>[7x]SAAWEDEDLDTDNDNIPDAYEKNGYTIKDSIAVKWNDSFAEQGYKKYVSSYLESNTAGDPYTDYQKASGSIDKAIKLEARDPLVAAYPVVGVGMENLIISTNEHASSDQGKTVSRATTNSKTDANTVGVSISAGYQNGFTGNITTSYSHTTDNSTAVQ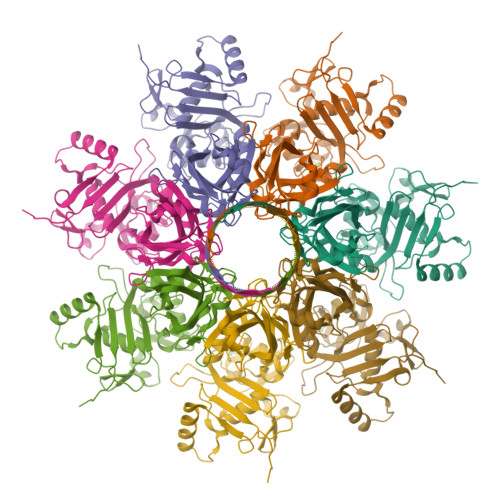DSNGESWNTGLSINKGESAYINANVRYYNTGTAPMYKVTPTTNLVLDGETLATIKAQDNQIGNNLSPNETYPKKGLSPLALNTMDQFNARLIPINYDQLKKLDSGKQIKLETTQVSGNYGTKNSQGQIITEGNSWSNYISQIDSVSASIILDTGSQTFERRVAAKEQGNPEDKTPEITIGEAIKKAFSATKNGELLYFNGIPIDESCVELIFDDNTSEIIKEQLKYLDDKKIYNVKLERGMNILIKVPSYFTNFDEYNNFPASWSNIDTKNQDGLQSVANKLSGETKIIIPMSKLKPYKRYVFSGYSKDPSTSNSITVNIKSKEQKTDYLVPEKDYTKFSYEFETTGKDSSDIEITLTSSGVIFLDNLSITELNSTPEILKEPEIKVPSDQEILDAHNKYYADIKLDTNTGNTYIDGIYFEPTQTNKEALDYIQKYRVEATLQYSGFKDIGTKDKEIRNYLGDQNQPKTNYINFRSYFTSGENVMTYKKLRIYAVTPDNRELLVLSVN5'-O-[(R)-(2-amino-1H-imidazol-1-yl)(hydroxy)phosphoryl]guanosine 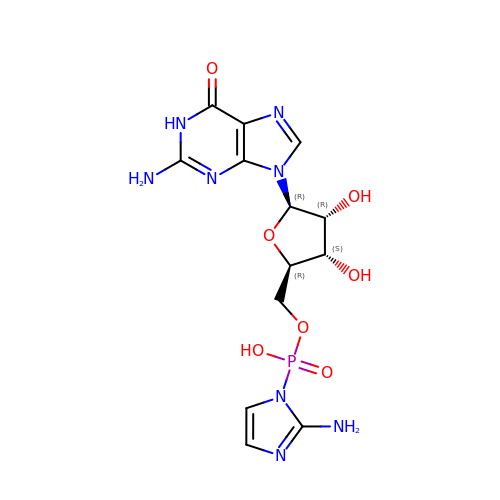| C13 H17 N8 O7 P | UJFHHYLHXPKINK-IOSLPCCCSA-N>[2x]GAMDPREVILCKDQDGKIGLRLKSIDNGIFVQLVQANSPASLVGLRFGDQVLQINGENCAGWSSDKAHKVLKQAFGEKITMTIRDRPFERTITMHKDSTGHVG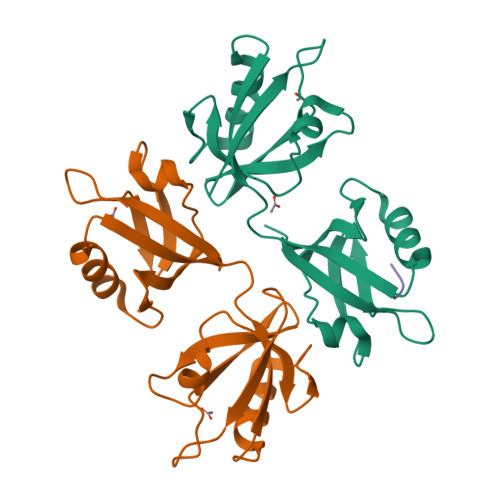FIFKNGKITSIVKDSSAARNGLLTEHNICEINGQNVIGLKDSQIADILSTSGTVVTITIMPAF;> ETLEDSVF> MNVPVGHLRNVQVLGIDAGGTMTDTFFVDQDGDFVVGKAQSTPQNEALGLIASSEDGLANWGMSLHEALAQLQTGVYSGTAMLNRVVQRKGLKCGLIVNRGMEDFHRMGRAVQSHLGYAYEDRIHLNTHRYDPPLVPRHLTRGVVERTDMMGTQVIPLREDTARDAARDLIAADAEGIVISLLHSYKNPVNERRVRDIVLEEVEKSGKKIPVFASADYYPVRKETHRTNTTILEGYAAEPSRQTLSKISNAFKERGTKFDFRVMATHGGTISWKAKELARTIVSGPIGGVIGAKYLGEVLGYKNIACSDIGGTSFDVALITQGEMTIKNDPDMARLVLSLPLVAMDSVGAGAGSFIRLDPYTRAIKLGPDSAGYRVGVCWKESGIETVTISDCHMVLGYLNPDNFLGGAVKLDRQRSVDAIKAQIADPLGLSVEDAAAGVIELLDSDLRDYLRSMI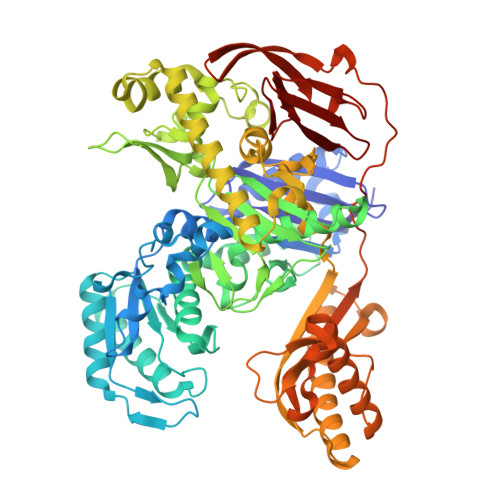SGKGYSPASFVCFSYGGAGPVHTYGYTEGLGFEDVIVPAWAAGFSAFGCAAADFEYRYDKSLDINMPTETPDTDKEKAAATLQAAWEELTKNVLEEFKLNGYSADQVTLQPGYRMQYRGQLNDLEIESPLAQAHTAADWDQLTDAFNATYGRVYAASARSPELGYSVTGAIMRGMVPIPKPKIPKEPEEGETPPESAKIGTRKFYRKKRWVDAQLYHMESLRPGNRVMGPAVIESDATTFVVPDGFETWLDGHRLFHLREV> AIVSSVDRKIFVLLRDGRMLFGVLRTFDQYANLILQDCVERIYFSEENKYAEEDRGIFMI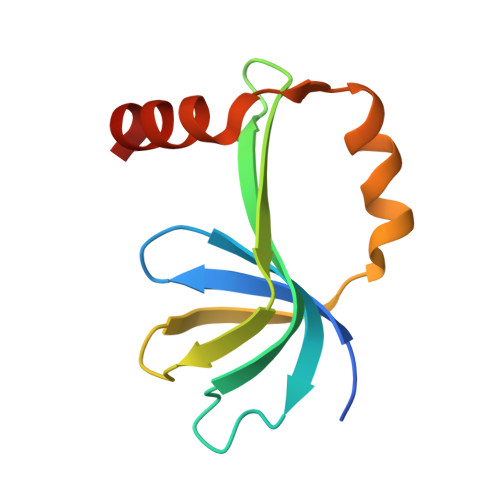RGENVVMLGEVDIDKEDQPLEAMERIPFKEAWLTKQKNDEK Bromomemantine | C12 H20 Br 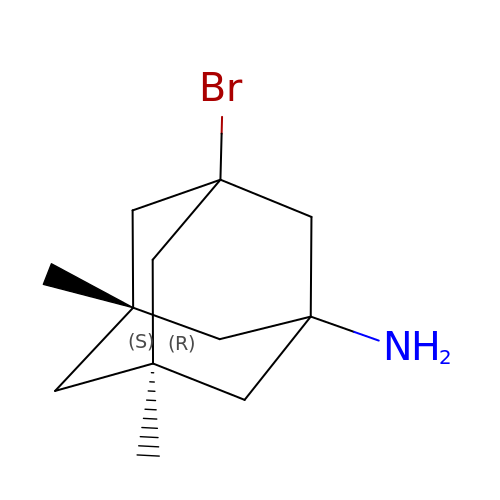N | UKCUZUGMIJFTKF-IWDIQUIJSA-N> MDAKKVAKKAAIQAARRITELAQVLVELLKEALKLDLTQEMRKKLIERYAAAIIRAIGDINNAIYQAKQEAEKLKKAGLVDSDQLDALL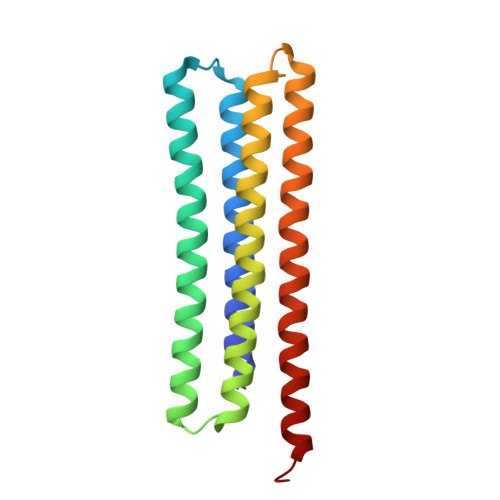RALDELQKVASKAANQLGRLFEEALKRLDKDNGGEEEKDRTAKWFEFEARAIEIALRLAAIGDVFDLEKEWRKLKSRGKL>[4x]MVAIVDVGITKFGKRKENIFDLVKEVTEKLLKYDIDYVIVSNSYSGEFNQTSGLSSL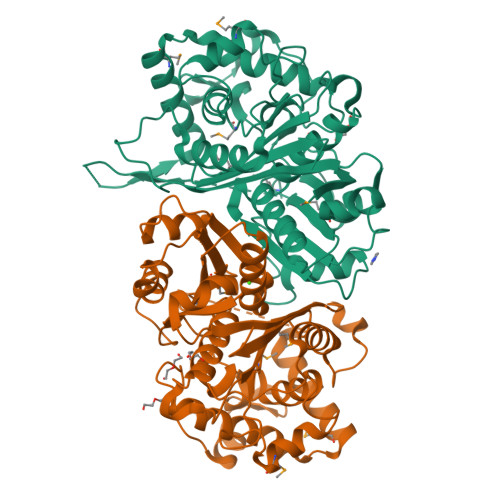ITTYLNLDYVPSLRVDNTSGSGGSAILVAKSLLESKEANTVLVVGVEKMSEKKTREVTKIISSLLPFEERIASLPSLASISAIEYMRKFNAPRESIAQVAVKNHYNGSLNPFAHIQKRVTLEEVLNSPVISEPLRLYEYTPISDGAAAVVMVRNEDALSYTSKPVYIKGIGSSNYTAYVSEKEDFVTLPAVVEASRKAFKKAKVERIDFAELHDMATILEIIQSEDIGLFKKGEGWKAVMEGLTSLDGEIPINPSGGLNSKGHPIGASGVAQAVEAFSQIRNEAGNRQVKNARVGLSLSMAGYGNSATVIIYGDEP> ATFEI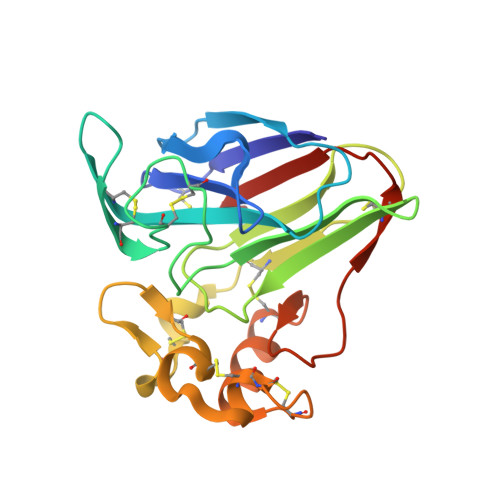VNRCSYTVWAAASKGDAALDAGGRQLNSGESWTINVEPGTNGGKIWARTDCYFDDSGSGICKTGDCGGLLRCKRFGRPPTTLAEFSLNQYGKDYIDISNIKGFNVPMNFSPTTRGCRGVRCAADIVGQCPAKLKAPGGGCNDACTVFQTSEYCCTTGKCGPTEYSRFFKRLCPDAFSYVLDKPTTVTCPGSSNYRVTFCPTA2-[[(4~{S})-5-chloranyl-6-methyl-1,2,3,4-tetrahydrothieno[2,3-d]pyrimidin-4-yl]sulfanyl]ethanoic 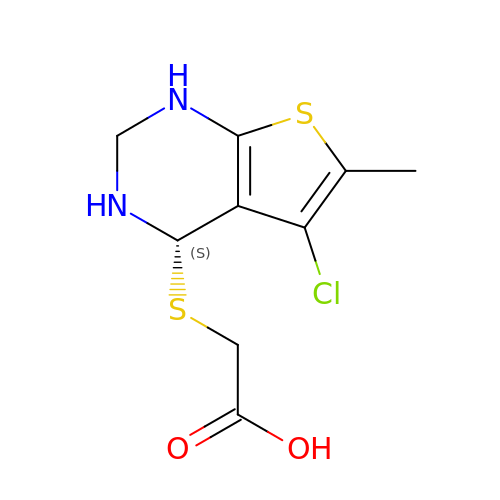acid | C9 H11 Cl N2 O2 S2 | YXTHLXJCVDULSY-QMMMGPOBSA-N>[2x]MKIRDLLKARRGPLFSFEFFPPKDPEGEEALFRTLEELKAFRPAFVSITYGAMGSTRERSVAWAQRIQSLGLNPLAHLTVAGQSRKEVAEVLHRFVESGVENLLALRGDPPRGERVFRPHPEGFRYAAELVALIRERYGDRVSVGGAAYPEGHPESESLEADLRHFKAKVEAGLDFAITQLFFNNAHYFGFLERARRAGIGIPI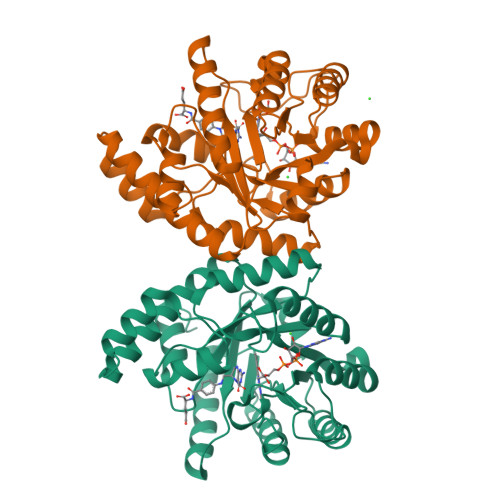LPGIMPVTSYRQLRRFTEVCGASIPGPLLAKLERHQDDPKAVLEIGVEHAVRQVAELLEAGVEGVHFYTLNKSPATRMVLERLGLRPASGQP>ASSWVMLGLLLSLLNRLSLAAEAYKKAIELDPNDALAWLLLGSVLLLLGREEEAEEAARKAIELKPEMDSARRLEGIIELIRRAREAAERAQEAAERTGDPRVR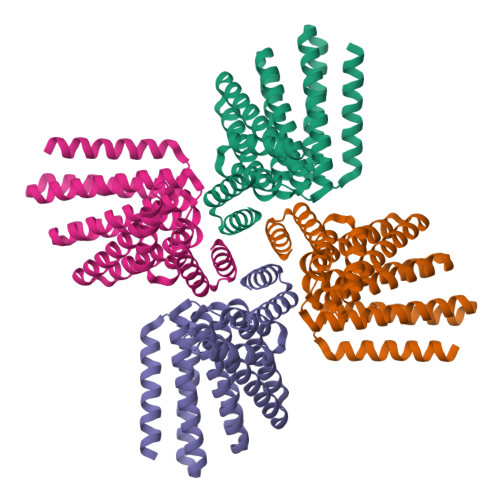ELARELKRLAQEAAEEVRRDPDSKDVNEALKLIVEAIEAAVRALEAAERTGDPEVRELARELVRLAVEAAEEVQRNPSSSDVNEALKLIVEAIDAAVRALEAAEKTGDPEVRELARELVRLAVEAAEEVQRNPSSEEVNEALKDIVKAIQEAVESL[4x]> MDFTSSSGVLDSERNTGSNDSDEPSSHSDVIETEELKLIKLQEHKNNLLRQRSELLDQLSQTRVVEPRSVQLDDKLLLKLLRRNDNAVSDSSQSSNNPLPRVLPSLNIEQRKKYLDITLNDVTVTCEKDMILLRKGSFTASFRIAVENESIRSMAIDLNAFEVELQPIIQYAEDTQNVNVAMMAVVQFLRIKELHEQMISKI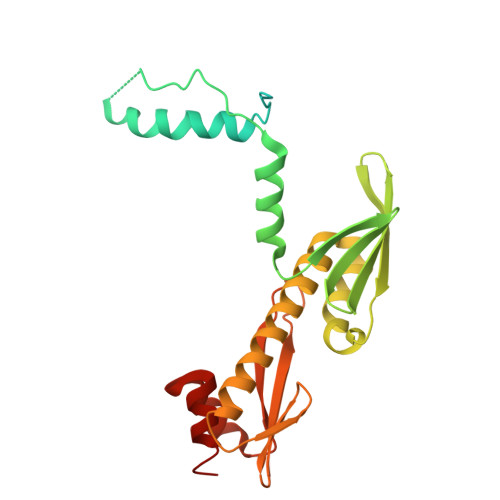VEASKFIRASNNTITLNDLEVSFHCYWNLPSPYPETLILTNKVQKILDFLIYQYGIQLGVIKYGSTII> MKNIKKNQVMNLGPNSKLLKEYKSQLIELNIEQFEAGIGLILGDAYIRSRDEGKTYCMQFEWKNKAYMDHVCLLYDQWVLSPPHKKERVNHLGNLVITWGAQTFKHQAFNKLANLFIVNNKKTIPNNLVENYLTPMSLAYWFMDDGGKWDYNKNSTNKSIVLNTQSFTFEEVEYLVKGLRNKFQLNCYVKINKNKPIIYIDSMSYLIFYNLIKPYLIPQMM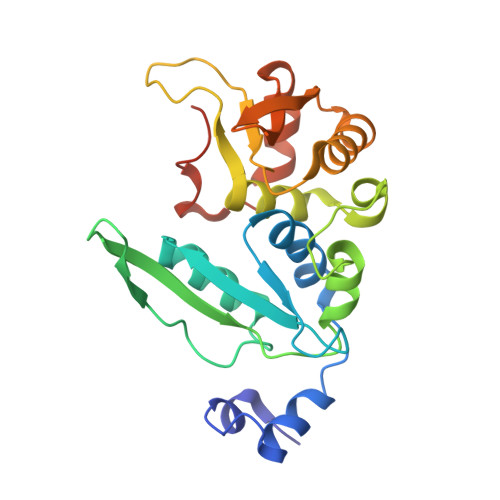YKLPNTISSETFLK>MRYVVGHKNPDTDSIASAIVLAYFLDCYPARLGDINPETEFVLRKFGVMEPELIESAKGKEIILVDHSEKSQSFDDLEEGKLIAIIDHHKVGLTTTEPILYYAKPVGSTATVIAELYFKDAIDLIGGKKKELKPDLAGLLLSAIISDTVLFKSPTTTDLDKEMAKKLAEIAGISNIEEFGMEILKAKSVVGKLKPEEIINMDFKNFDFNGKKVGIGQVEVIDVSEVESKKEDIYKLLEEKLK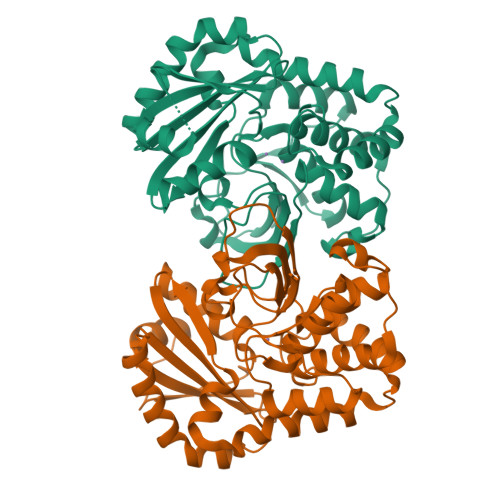NEGYDLIVFLITDIMKEGSEALVVGNKEMFEKAFNVKVEGNSVFLEGVMSRKKQVVPPLERAYNG[2x]RIBOSE-5-PHOSPHATE | C5 H11 O8 P | 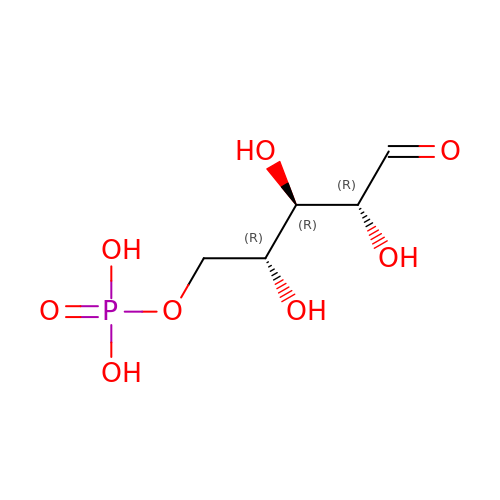PPQRONHOSHZGFQ-LMVFSUKVSA-N>MSVTRRELLKLAGAAGAMSLAPAIVRAQKLEKAKVQIAVGGKPLIYYLPLTIAEVKGFFKDEGLDVSIADFAGGSKALQAVVGGSADVVSGAFEHTLSLQAKGQFYRAFALQGRAPMIGVGVSKKNLPGYKGPADLKGRKIGVTAPGSSTNMVVNFFLAKHGLKASDVSFIGVGAGAGAVTALRSGQIDAISNTDPVVSMLETSGDIQIIVDTRTLKDTKEIFGGNMPAGCLYAPQAFVDANPNTAQALTNAIVRADKWIQKAGADEIAKAVPEGYLLGDPAVYKAAIGKSMEGLS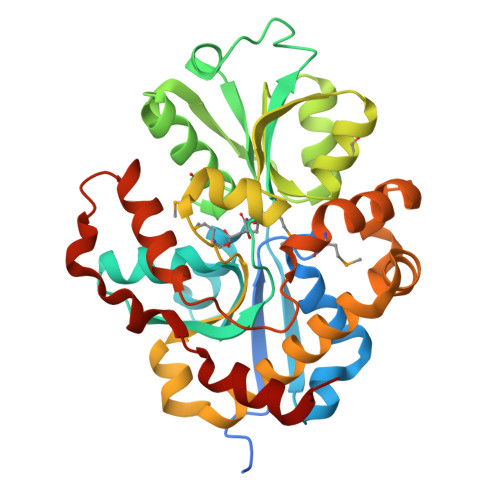PDGVIPEDGAATALKALAAFVPDFDAAKVDPAKAWTNEYTRRANEKYPNG[2x]> GPAPHEERVGDMRIVNITFSDINSIKNFQPFSQYFDFTLTGPRYNGNIAQFAMIWKIKNPPHNLLGVFFDNNTRDDEDDKYTLEEL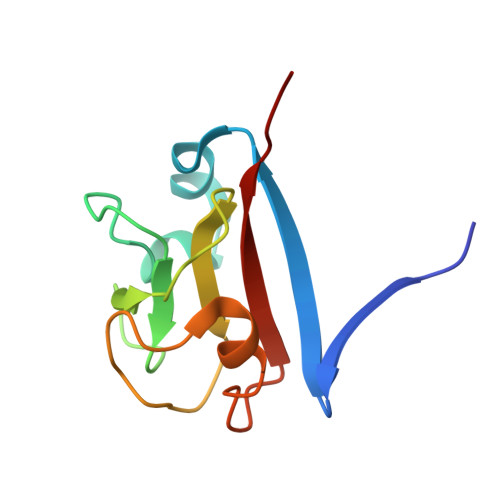KQMGNGAKNMYIFWQYEQK>ALAIAAVNAVTGEVDKLSDRVVALEVAVNGGTQVAVREFDMAAELLMRQLLKLDGIEAEGDAKVQRKAEVRRIQNLQEAVD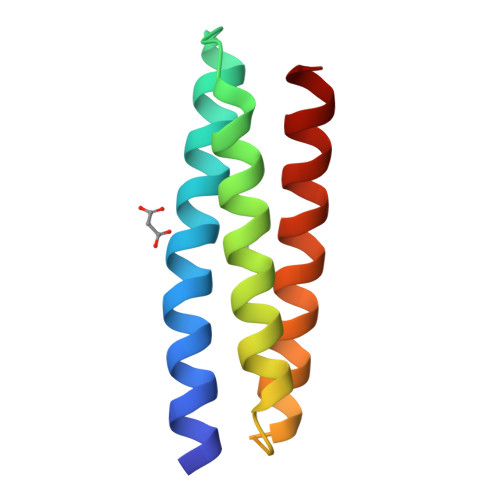KLKARCS[5x]Phytochromes are red-light photoreceptors found in various plants and microorganisms. S. aurantiaca contains two previously uncharacterized bacteriophytochromes (BphPs) denoted SaBphP1 and SaBphP2, which may be responsible for the light-stimulated growth of multicellular fruiting bodies. The classical BphPs switch between a red absorbing state denoted Pr (λmax ≃ 700 nm) and a far-red absorbing state denoted Pfr (λmax ≃ 750 nm).

In order to understand the role of the unusual Thr289 in signal transduction in SaBphP1, we replaced it with a His so that the T289H variant SaBphP1 resembles classical BphPs. The mutant PCM also crystallizes in the dark in the Pr state in P3221 with three subunits denoted A, B and C in the asymmetric unit, but the PCM-wt crystallized in space group C2 with a single, dimeric BphP molecule in the asymmetric unit. In the mutant PCM crystals, subunits A and B form a non-crystallographic dimer, and the third subunit, C, is related to its mate through a crystallographic twofold symmetry. Interestingly, the crystallization conditions for the PCM wild-type and T289H mutant are the same, yet they crystallize in different space groups. This already suggests that the mutation affects the relative domain orientation. Indeed, the r.m.s.d. between the T289H mutant and wild-type PCM is ∼3 Å overall. As shown in Fig. 5(b) and Table 2, the PAS and GAF domains superimpose well, but the PHY domains occupy different positions. PHY displacements between the wild-type and T289H mutant are on the order of 4 Å. It demonstrates how tightly the PHY domain is coupled to the structural state of the BV chromophore and its immediate environment, a coupling that is essential to a signaling protein.

>MSTEASRSGKQEVDLTNCDREPIHIPGAIQPHGVLLVLSEPGLVLTHASENAPAVLGNSAEQLLGAPLGHFIEPSVREPLEADLRSARLKQLNPLKVVWRVDGVDRFFDGIAHRHQGRLILELEPSSHREAVPFLSFFHAVRDGLSRLRDARDLQELCEAVVQEVRGLTGFDRAIIYRFDAEWNGSVIAEARDARADPYLGLHFPASDIPRQARELYQLNWLRIIPTIDYQPARVRALPGHGEPLDLSFSVLRSVSPIHLEYLHNMGVQASMSISLMKDGKLWGLISCHQVSGTRYVPYEVRTACEFLGEVMSSLLAAKEGNEDYDQRIRAKSIHAALLERMAREVDFVSGLASQESGLLELVHAHGAAIHFHGRTTVLGQAPSDEALTGLIEWLGSRTGEGVFCTDRLAREYPEAQAFQEVAAGLMAFSMSRGRNNFVLWFRPEAVQTVNWSGNPTKAVEFDQGGPRLHPRKSFELWKETVRGRCLPWKAYEVEAASELRRSIIDVALQRSEEL[3x]> TLSILVAHDLQRVIGFENQLPWHLPNDLKHVKKLSTGHTLVMGRKTFESIGKPLPNRRNV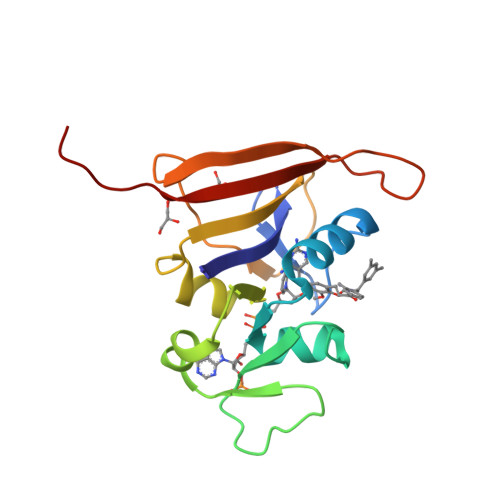VLTSDTSFNVEGVDVIHSIEDIYQLPGHVFIFGGQTLFEEMIDKVDDMYITVIEGKFRGDTFFPPYTFEDWEVASSVEGKLDEKNTIPHTFLHLIRKKLVPR>[4x]MST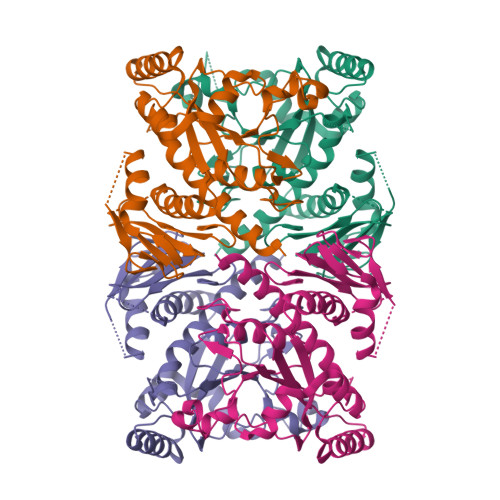FGKLFRVTTYGESHCKSVGCIVDGVPPGMSLTEADIQPQLTRRRPGQSKLSTPRDEKDRVEIQSGTEFGKTLGTPIAMMIKNEDQRPHDYSDMDKFPRPSHADFTYSEKYGIKASSGGGRASARETIGRVASGAIAEKFLAQNSNVEIVAFVTQIGEIKMNRDSFDPEFQHLLNTITREKVDSMGPIRCPDASVAGLMVKEIEKYRGNKDSIGGVVTCVVRNLPTGLGEPCFDKLEAMLAHAMLSIPASKGFEIGSGFQGVSVPGSKHNDPFYFEKETNRLRTKTNNSGGVQGGISNGENIYFSVPFKSVATISQEQKTATYDGEEGILAAKGRHDPAVTPRAIPIVEAMTALVLADALLIQKARDFSRSVVHHHHHHH>[3x]AQVINTFDGVADYLQTYHKLPDNYITKSEAQALGWVASKGNL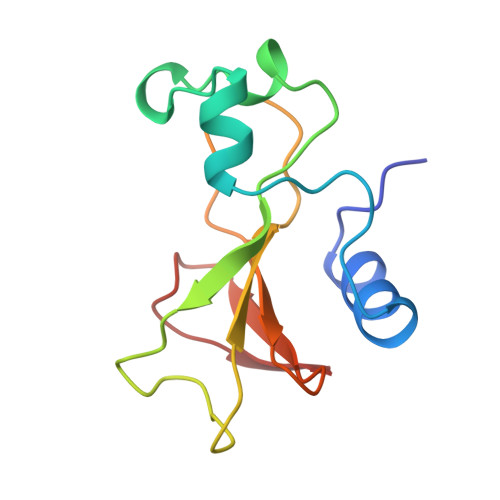ADVAPGKSIGGDIFSNREGKLPGKSGSTWREADINYTSGFRNSDRILYSSNWLIYKTTDHYQTFTKIR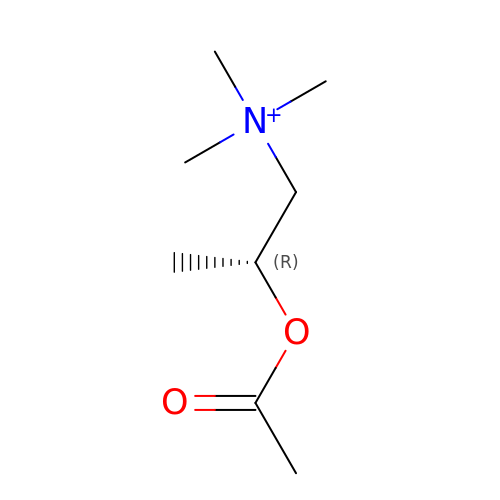[(2R)-1-(trimethyl-$l^4-azanyl)propan-2-yl] ethanoate | C8 H18 N O2 | TXPWCDJHFBRHES-SSDOTTSWSA-N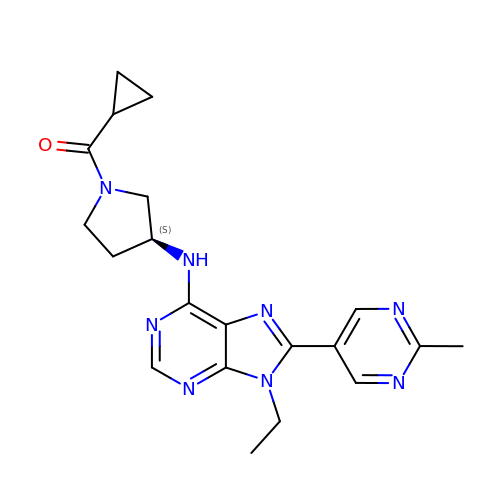cyclopropyl[(3S)-3-{[9-ethyl-8-(2-methylpyrimidin-5-yl)-9H-purin-6-yl]amino}pyrrolidin-1-yl]methanone | C20 H24 N8 O | DADGJAZOHPBTCZ-HNNXBMFYSA-N>[2x]EQIRYKIPEEMPTGSVVGNLAKDLGFSVQELPTRKLRISSEKPYFSVSSESGELLVSSRLDREQICGKKLMCALEFEAVAENPLNFYHLSVELEDINDHTPKFAHTSFELQISESSKPGTRFILGSAHDADIGTNSLQNYQLSPNDHFSLVNKEKSDGSKYPEMILKTALDREKQKLYHLTLTALDFGHPPLNSTAQIQVLVTDANDNPPVFSQDIYRVSLPENVYPGTTVLRVVATDQDEGVNSEITFSFSEAGQVTQFNLDSNTGEITTLHTLDFEEVKEYSLVLEAKDGGGMIAQCTVEIEVLDENDNVPEVLFQSLPDLIMEDAEPGTYIALLKTRDKDSGRNGEVICKLEGGAPFK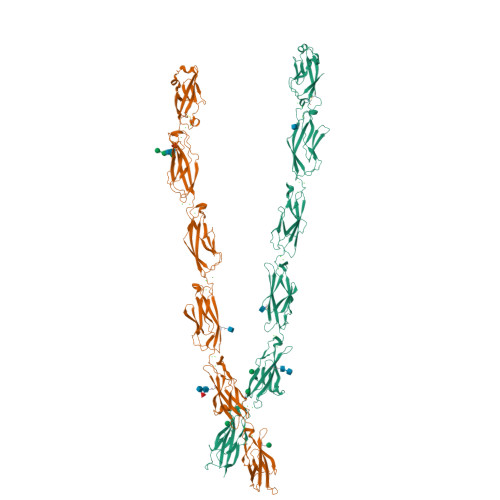ILTSSGNTYKLVTDGVLDREQNPEYNITIRATDKGDPPLSSSSSVTLHIGDVNDNAPVFTKVSYLVHVAENNPPGASIAQVSASDPDLGANGQVTYYIIASDLEPESLWSYVTINAQSGVLFAQRAFDHEQLRSFQLTLQARDHGSPTLSANVSMRLLVGDRNDNAPRVLYPTLEPDGSALFDMVPRSAEPGYLVTKVVAVDADSGHNAWLSYHVLQASDPGLFSLGLRTGEVRTARALGDRDSARQRLLVAVRDGGQPPLSATATLHLIFADSLQEHHHHHHHH>GSSLENLPPVAASIEQLLERQWSEGQQFLLEQGTPSDILGMLKSLHQLQVENRRLEEQIKNLTAKKERLQLLNAQLS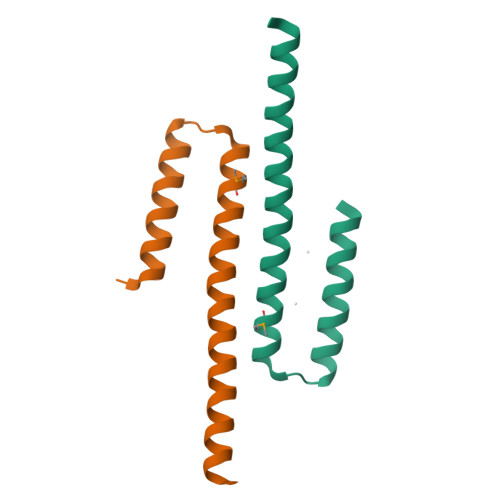[2x]>[2x]GPLGSGEPGSARAAVSELMQLFPRGLFEDALPPIVLRSQ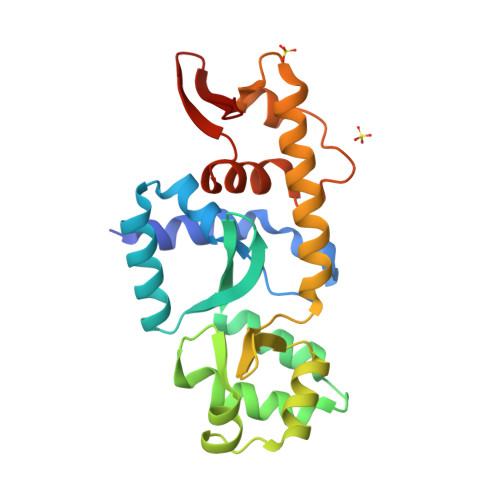VYSLVPDRTVADRQLKELQEQGEIRIVQLGFDLDAHGIIFTEDYRTRVLKASDGRPYAGAVQKFLASVLPASGDLSFQQDQMTQTFGFRDSEITHLVNAGVLTVRDAGSWWLAVPGAGRFIKYFVKGRQAVLSMVRKAKYRELLLSELLGRRAPVVVRLGLTYHVHDLIGAQLVDSISTTSGTLLRLPET> EPEITLIIFGVIAGVIG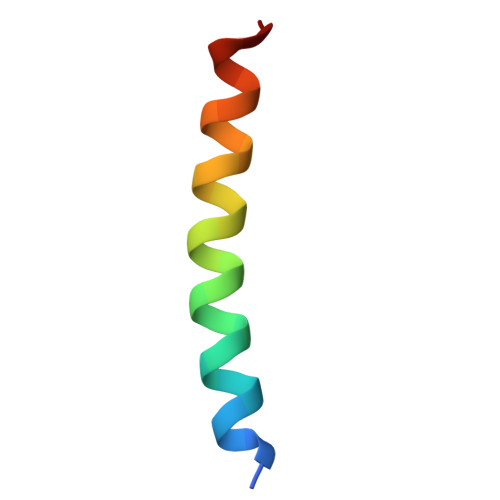TILLISYGIRRLC>[2x]MADDQGCIEEQGVEDSANEDSVDAKPDRSSFVPSLFSKKKKNVTMRSIKTTRDRVPTYQYNMNFEKLGKCIIINNKNFDKVTGMGVRNGTDKDAEALFKCFRSLGFDVIVYNDCSCAKMQDLLKKASEEDHTNAACFACILLSHGEENVIYGKDGVTPIKDLTAHFRGDRCKTLLEKPKLFFIQACRGTELDDGIQAD;>SGPINDTDANPRYKIPVEADFLFAYSTVPGYVSYRVPGRGSWFVQ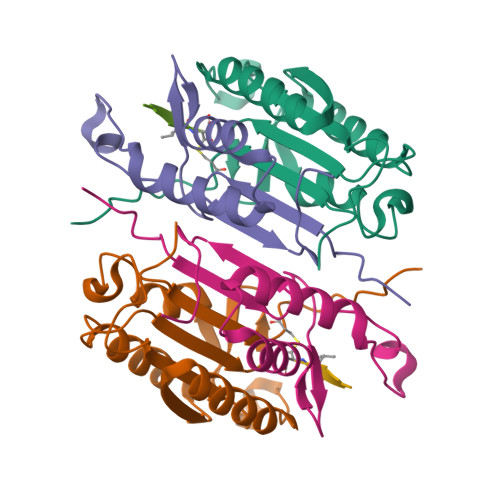ALCSILEEHGKDLEIMQILTRVNDRVARHFESDSDDPHFHEKKQIPCVVSMLTKELYFSQLEHHHHHH[2x]5-{[(2-aminoethyl)sulfanyl]methyl}furan-2-carbaldehyde | C8 H11 N O2 S | 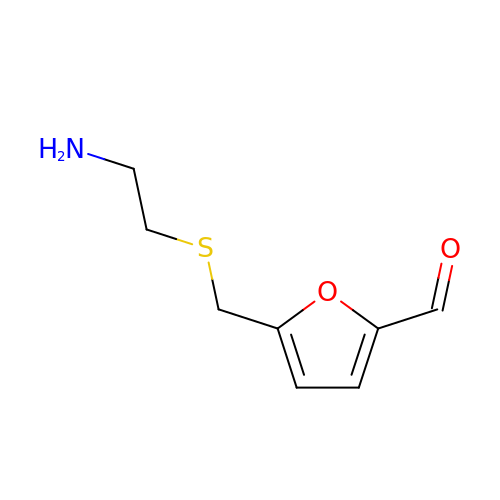IXLKFYGLYDVEMS-UHFFFAOYSA-N>[4x]APAPQPPPILKVFNRPILFDIVSRGSTADLDGLLSFLLTHKKRLTDEEFREPSTGKTCLPKALLNLSNGRNDTIPVLLDIAERTGNMREFINSPFRDIYYRGQTSLHIAIERRCKHYVELLVAQGADVHAQARGRFFQPKDEGGYFYFGELPLSLAACTNQPHIVNYLTENPHKKADMRRQDSRGNTVLHALVAIADNTRENTKFVTKMYDLLLLKCSRLFPDSNLETVLNNDGLSPLMMAAKTGKIGVFQHIIRREVTDEDTRHLSRKFKDWAYGPVYSSLYDLSSLDTCGEEVSVLEILVYNSKIENRHEMLAVEPINELLRDKWRKFGAVSFYINVVSYLCAMVIFTLTAYYQPLEGTPPYPYRTTVDYLRLAGEVITLFTGVLFFFTSIKDLFTKKCPGVNSLFVDGSFQLLYFIYSVLVVVSAALYLAGIEAYLAVMVFALVLGWMNALYFTRGLKLTGTYSIMIQKILFKDLFRFLLVYLLFMIGYASALVTLLNPCTNMKVCDEDQSNCTVPTYPACRDSETFSAFLLDLFKLTIGMGDLEMLSSAKYPVVFILLLVTYIILTFVLLLNMLIALMGETVGQVSKESKHIWKLQWATTILDIERSFPVFLRKAFRSGEMVTVGKSSDGTPDRRWCFRVDEVNWSHWNQNLGIINEDPGK

The transient receptor potential vanilloid 4 (TRPV4) channel is a polymodal receptor that is activated by warm temperature, osmolarity changes, and many ligands. Like other members in the TRPV family, TRPV4 is critically involved in a plethora of physiological processes like temperature sensation, osmoregulation, and mechanotransduction. To understand how the TRPV4 channel is activated and inhibited by ligands and to facilitate drug development targeting this channel in the future, we have resolved the structures of mouse TRPV4 in the apo state (mTRPV4apo, 3.6 Å), in complex with the agonist GSK1016790A (GSK101) (mTRPV4GSK101, 3.6 Å), in complex with both GSK101 and ruthenium red (RR) (mTRPV4GSK101_RR, 3.7 Å) and in complex with Agonist-1 and RR (mTRPV4Agonist1_RR, 3.9 Å) states by cryo-electron microscopy (cryo-EM). In summary, we have identified the cytosol-facing cavity in the S1 to S4 bundle as a hot spot for GSK101 and Agonist-1 binding in TRPV4.

We first observed that mTRPV4apo is a homotetramer, where the S1 to S4 bundle and pore domain composed of S5 and S6 are organized in a domain-swapped manner. The mTRPV4apo is in a closed state, with the residue M718 forming the permeation-restricting site in S6. The selectivity filter of mouse TRPV4 adopts an open conformation in the apo state, which is distinct from those in TRPV1 or TRPV2. Moreover, though the subunit in both xTRPV4 and mTRPV4 is domain-swapped, the pore domain in xTRPV4 locates much closer to the S1 to S4 bundle as compared to those in mTRPV4 (subunits in green and tan, respectively). Therefore, we believe that the structure of xTRPV4 is less relevant when the function of TRPV4 is considered in mammals.> VNQSETEIEILAEKIARWARARSAEIERDRRLPDELVTRLREAGLLRATMPREVAAPELAPGRALRCAEAVARGDASAGWCVSIAITSALLVAYLPARSREEMFGGGRGVAAGVWAPRGTARSVDGGVVVSGRWPFCSGINHADIMFAGCFVDDRQVPSVVALNKDELQVLDTWHTLGLRGTGSHDCVADDVFVPADRVFSVFDGPIVDRPLYRFPVFGFFALSIGAAALGNARAAIDDLVELAGGKKGLGTTRTLAERSATQAAAATAESALGAARALFYEVIEAAWQVSHDAEAVPVTMRNRLRLAATHAVRTSADVVR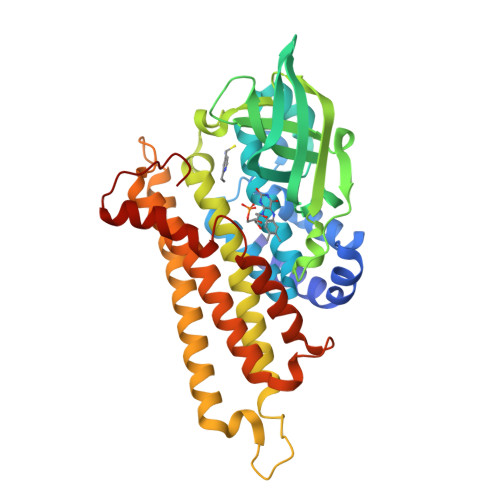SMYDLAGGTAIYDNAPLQRRFRDAFTATAHFQVNEASRELPGRVLLDQPADVSML> M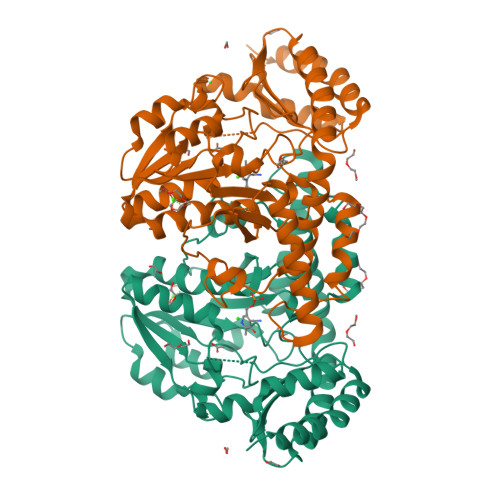AYFDYTSAKPVDERILEAMLPYMTESFGNPSSVHSYGFKAREAVQEAREKVAKLVNGGGGTVVFTSGATEANNLAIIGYAMRNARKGKHILVSAVEHMSVINPAKFLQKQGFEVEYIPVGKYGEVDVSFIDQKLRDDTILVSVQHANNEIGTIQPVEEISEVLAGKAALHIDATASVGQIEVDVEKIGADMLTISSNKIYGPKGVGALWIRKEAKLQPVILGGGQENGLRSGSENVPSIVGFGKAAEITAMEWREEAERLRRLRDRIIDNVLKIEESYLNGHPEKRLPNNVNVRFSYIEGESIVLSLDMAGIQASTGSACSSKTLQPSHVLMACGLKHEEAHGTLLLTLGRYNTDEDVDRLLEVLPGVIERLRSMSPLYRR> MGIDINTKIFNSVAEVFQKAQGSYAGHRKHIAVLKKIQSKAVEQGYEDAFNFWFDKLVTKILPLKKNEIIGDRIVKLVAAFIASLERELILAKKQNYKLTNDEEGIFSRFVDQFIRHVLRGVESPDKNVRFRVLQLLAVIMDNIGEIDESLFNLLILSLNKRIYDREPTVRIQAVFCLTKFQDEEQTEHLTELSDNEENFEATRTLVASIQNDPSAEVRRAAMLNLINDNNTRPYILERARDVNIVNRRLVYSRILKSMGRKCFDDIEPHIFDQLIEWGLEDRELSVRNACKRLIAHDWLNALDGDLIELLEKLDVSRSSVCVKAIEALFQSRPDILSKIKFPESIWKDFTVEIAFLFRAIYLYCLDNNITEMLEENFPEASKLSEHLNHYILLRYHHNDISNDSQSHFDYNTLEFIIEQLSIAAERYDYSDEVGRRSMLTVVRNMLALTTLSEPLIKIGIRVMKSLSINEKDFVTMAIEIINDIRDDDIEKQESESDIINNLPPEKEASSATIVLCLTRSSYMLELVNTPLTENILIASLMDTLITPAVRNTAPNIRELGVKNLGLCCLLDVKLAIDNMYILGMCVSKGNASLKYIALQVIVDIFSVHGNTVVDGEGKVDSISLHKIFYKVLKNNGLPECQVIAAEGLCKLFLADVFTDDDLFETLVLSYFSPINSSNEALVQAFAFCIPVYCFSHPAHQQRMSRTAADILLRLCVLWDDLQSSVIPEVDREAMLKPNIIFQQLLFWTDPRNLVNQTGSTKKDTVQLTFLIDVLKIYAQIEKKEIKKMIITNINAIFLSSEQDYSTLKELLEYSDDIAENDNLDNVSKNALDKLRNNLNSLIEEINERSETQTKDENNTANDQYSSILGN;> GPLGHMSIFEKDLMAYFDENLNRNWRGREHWKVRNFKKANKSMDTKKKHKQKKVLEIDFFKTDDSFEDKVFASKGRTKIDMPIKNRKNDTHYLLPDDFHFSTDRITRLFIKPGQKMSLFSHRKHT

Condensin protein complexes coordinate the formation of mitotic chromosomes and thereby ensure the successful segregation of replicated genomes. Here, we identify a direct DNA-binding site in the eukaryotic condensin complex, which is formed by its Ycg1Cnd3 HEAT-repeat and Brn1Cnd2 kleisin subunits. A peptide loop of the kleisin subunit encircles the bound DNA and, like a safety belt, prevents its dissociation. Firm closure of the kleisin loop around DNA is essential for the association of condensin complexes with chromosomes and their DNA-stimulated ATPase activity.

Even in the co-crystal structures of Sc Ycg1–Brn1 with DNA, 43 residues of the linker that connects the α1 and α2 segments of Brn1 remained disordered. The trajectories of the visible residues that flank the linker, however, indicate that the path of the connecting peptide leads over the bound DNA helix. Since the length of this linker is considerably shorter in most other species, we shortened the linker of Sc Brn1 by 27 residues to match the linker length of the human NCAPH kleisin subunit and co-crystallized the new construct with DNA. The structure of this construct very closely resembles the previous Sc Ycg1–Brn1–DNA structures. Although the shortened linker also remained disordered in this structure, the only conceivable way to span the distance of ∼36 Å between the two visible ends with the short linker is by running the connecting peptide over the DNA helix. As a consequence, the Brn1 kleisin subunit encircles the DNA double helix within the loop that is formed by the association of its N-terminal latch and C-terminal buckle segments. Furthermore, addition of BMOE created a crosslink of the Brn1 loop and resulted in the formation of an SDS-resistant complex with circular DNA substrates even in the context of the Ct Ycs4–Ycg1–Brn1 ternary complex. These experiments provide proof that the DNA bound within the Ycg1–Brn1 groove must be enclosed by the Brn1 loop.> MTIDQKNTNIDPRFPHHHPRPQSFWEARAKALESLLIEKGHLSSDAIERVIKH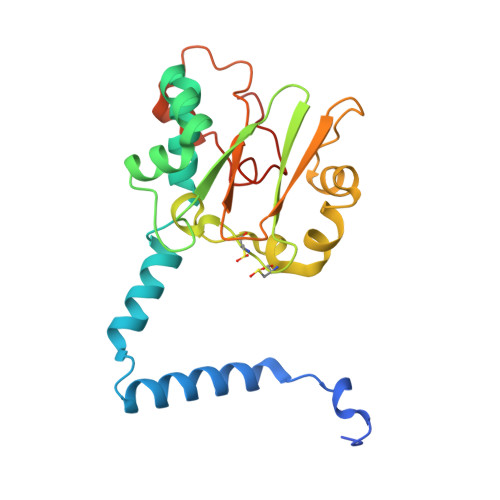YEHELGPMNGAKVVAKAWTDPAFKQRLLEDSETVLRELGYYGLQGEHIRVVENTDTVHNVVVCTLCSCYPWPLLGLPPSWYKEPAYRARVVKEPRQVLKEFGLDLPDSVEIRVWDSSSEIRFMVLPQRPEGTEGVTEEELAKLVTRDSMIGVAKIEPPKVTVG N-[(cyclopentyloxy)carbonyl]-3-methyl-L-valyl-(4R)-N-[(1R,2S)-2-ethenyl-1-{[(1-methylcyclopropyl)sulfonyl]carbamoyl}cyclopropyl]-4-{[7-methoxy-3-(propan-2-yl)quinoxalin-2-yl]oxy}-L-prolinamide | C39 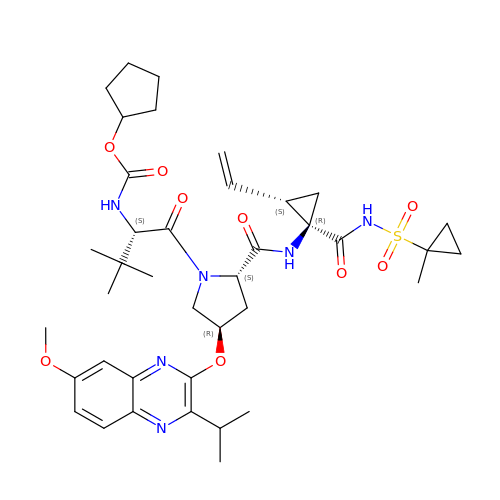H54 N6 O9 S | SXDJYVUXIXGZPI-GQBWDAOWSA-N> GASLKEIIDELGKQAKEQNKIASRILKIKGIKRIVVQLNAVPQDGKIRYSM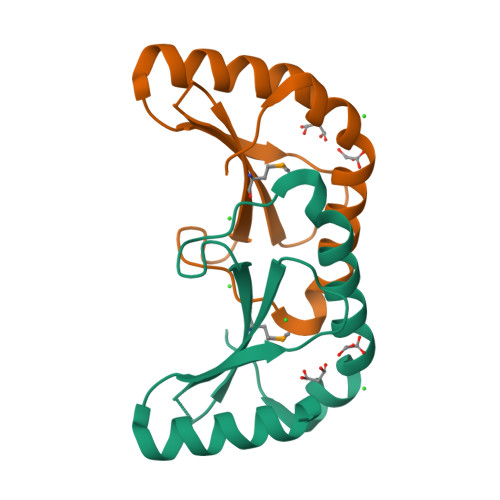TIHSQNNFRKQIGITPQDAEDLKLIAEFLEKYSDFLNEYVKFTPR(2~{R},3~{S},4~{S},5~{R},6~{R})-2-(hydroxymethyl)-6-[3-[(~{E})-2-(4-hydroxyphenyl)ethenyl]-5-oxidanyl-phenoxy]oxane-3,4,5-triol 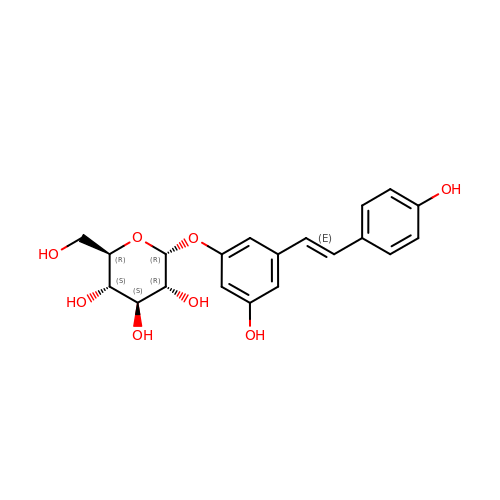| C20 H22 O8 | HSTZMXCBWJGKHG-UABZBGRASA-N>[2x]TPEMPVLENRAAQGDITAPGGARRLTGDQTAALRDSLSDKPAKNIILLIGDGMGDSEITAARNYAEGAGGFFKGIDALPLTGQYTHYALNKKTGKPDYVTDTAASATAWSTGVKTYNGALGVDIHEKDHPTILEMAKAAGLATGNVSTAELQDATPAALVAHVTSRKCYGPSATSEKCPGNALEKGGKGSITEQLLNARADVTLGGGAKTFAETATAG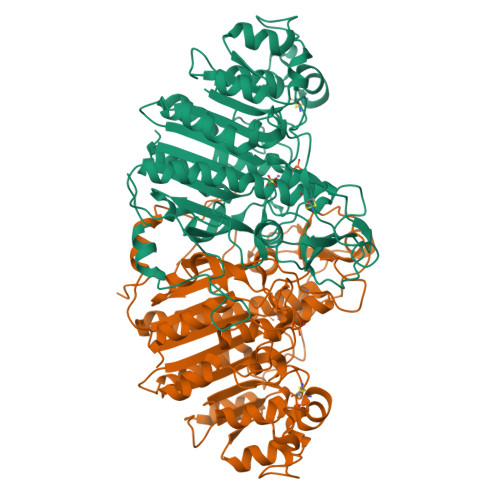EWQGKTLREQAQARGYQLVSDAASLNSVTEANQQKPLLGLFADGNMPVRWLGPKATYHGNIDKPAVTCTPNPQRNDSVPTLAQMTDKAIELLSKNEKGFFLQVEGASIDKQDHAANPCGQIGETVDLDEAVQRALEFAKKEGNTLVIVTADHAHASQIVAPDTKAPGLTQALNTKDGAVMVMSYGNSEEDSQEHTGSQLRIAAYGPHAANVVGLTDQTDLFYTMKAALGLK>[3x]MTSKREKSLDHTLELKIPFETER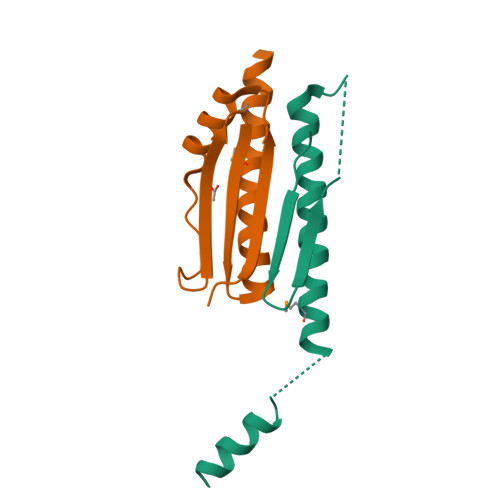QATIATKVLSPDPILKPQDFQVDYSSEKNVMLVQFRSIDDRVLRVGVSSIIDSIKTIVEAMDVLSHHHHHH;>MKLPVAQYSAPDGVEKSFAPIRDDPRYMTTEGRTTGPSDHVLNAGQIDRDKPSEPERTKDGSQLTYLGQLRTQLTGLQDDINEFLTGRMELAKNKKKAGADEKRIQEEINQLLDGGDGDEDAV[3x]> TIDTCSSDSPLSCQTDNEASCCFNSPGGSLLQTQFWDYDPSDGPSDSWTIHGLWPDNCDGTYQEYCDESREYSNITSILEAQNRTELLSYMKEYWPDYEGADEDESFWEHEWNKHGTCINTIEPSCYTDYYAQEEVGDFFQQVVDLFKTLDSYTALSDAGITPSEDATYKLSDIEDALAAIHDGYPPYVGCEDGALSQLYYYFNVKGSAIGGTYVASERLED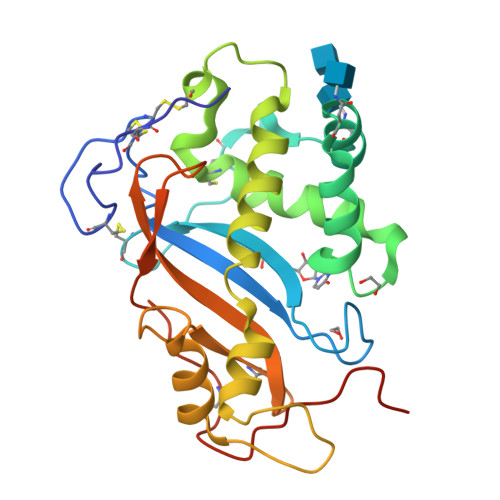SNCKDSGIKYPPKYSSSKKIYGSSL>[2x]AAKYAVVLKTLTDPFWVNMKKGIEDEAKKLGVSVDIFAAASEG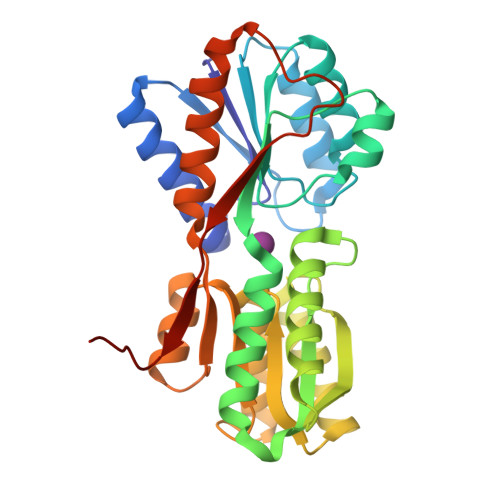DAEAQKSLFESLSNKNYKGIAFAPLTKDNLVEPVAAAWKKGTYLVNLDEKIDMKKLKAAGGAVEAFVTTDNVQVGAQGAGYIVQKLGAQGGEVAIIEGEAGNASGEARRTGATDQFAKASNIKLVASQPADWDRTKAKQVATEILAKNPNIKAIYCANDTMALGVADAVADAGKTGKVLVVGTDGIPEAQEAVKAGKMTATVAQNPAAIGATGLKLMVDAEKKGKVIPLDKAPQYVLVASKLVTALEHHHHHH> MAQNLKDLAGRLPAGPRGMGTALKLLLGAGAVAYGVRESVFTVEGGHRAIFFNRIGGVQQDTI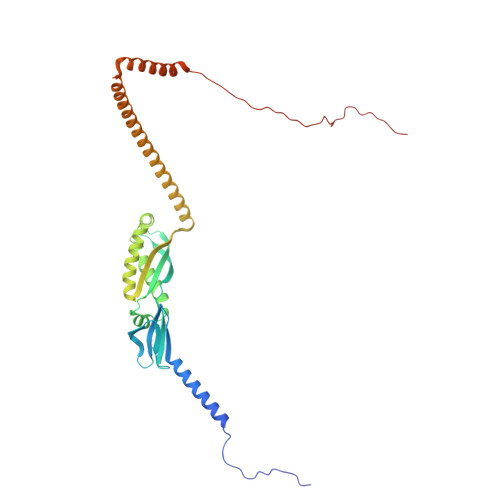LAEGLHFRIPWFQYPIIYDIRARPRKISSPTGSKDLQMVNISLRVLSRPNAQELPSMYQRLGLDYEERVLPSIVNEVLKSVVAKFNASQLITQRAQVSLLIRRELTERAKDFSLILDDVAITELSFSREYTAAVEAKQVAQQEAQRAQFLVEKAKQEQRQKIVQAEGEAEAAKMLGEALSKNPGYIKLRKIRAAQNISKTIATSQNRIYLTADNLVLNLQDESFTRGSDSLIKGKK> IDPRFPHH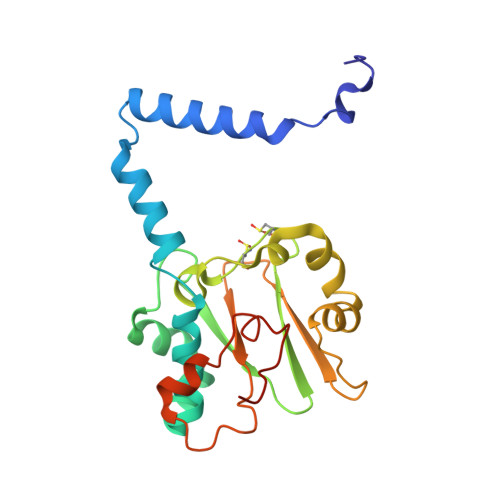HPRPQSFWEARAKALESLLIEKGHLSSDAIERVIKHYEHELGPMNGAKVVAKAWTDPAFKQRLLEDSETVLRELGYYGLQGEHIRVVENTDTVHNVVVCTLCSCYPWPLLGLPPSWYKEPAYRARVVKEPRQVLKEFGLDLPDSVEIRVWDRSSEIRFMVLPQRPEGTEGMTEEELAKLVTRDSMIGVAKIEPPKVTVG Bacteria harboring β-lactamase enzymes [E.C. 3.5.2.6] pose a significant threat to public health. These enzymes prevent β-lactam antibiotics from reaching their intended target, the penicillin binding proteins (PBPs). Sulbactam, tazobactam and clavulanic acid are mechanism-based inactivators as they share similarities with the β-lactam structure, the normal substrate for β-lactamases. Similar to a substrate, these inhibitors can, after acylation at catalytic residue S70, undergo several inhibitory reaction pathways including fragmentation in the active site and covalently cross-linking at S130.

Lastly, we changed the position of the ester bond, shortening the tail, and replaced the terminal carboxylate group with an amine group to result in PSR-3-226. PSR-3-226 was also not able to be trapped in the wt SHV-β-lactamase; we suspect that the tail of PSR-3-226 is not capable of forming a trans-enamine stabilizing U-shaped conformation. This prompted us to use the deacylation-deficient E166A variant of SHV-1 as we had done previously with difficult to capture compounds. Soaking E166A SHV-1 crystals for 30 minutes with PSR-3-226 yielded a 1.22Å resolution acyl-enzyme structure. Fo-Fc and 2Fo-Fc electron maps and subsequent crystallographic refinement indicated the presence of a covalently-bound partial PSR-3-226 fragment (refined at 100% occupancy) and a nearby HEPES buffer molecule fragment (refined at 80% occupancy). The PSR-3-226 inhibitor fragment, which consists of six atoms, was covalently bound to S70 in a trans-enamine conformation (torsion angle of 175°). Since only six atoms of the inhibitor fragment were able to be resolved, there were few hydrogen bonds observed in the active site; the inhibitor carbonyl oxygen occupied the oxyanion hole, as in SA2-13- and PSR-4-157-bound SHV-1, within hydrogen bonding distance of the mainchain nitrogens of residues A237 and S70. The one exception was residue 166, which was substituted to an alanine from glutamate to capture the inhibitor intermediate. This E166A change resulted in a local distortion of the main chain for this residue similar to what we observed previously for deacylation-deficient E166A inhibitor complexes. Interestingly, PSR-3-226 in both SHV-1 and KPC-2 is accompanied by a nearby buffer molecule interacting in the carboxyl binding pocket.

> SPQPLEQIKLSESQLSGRVGMIEMDLASGRTLTAWRADERFPMMSTFKVVLCGAVLARVDAGDEQLERKIHYRQQDLVDYSPVSEKHLADGMTVGELCAAAITMSDNSAANLLLATVGGPAGLTAFLRQIGDNVTRLDRWATELNEALPGDARDTTTPASMAATLRKLLTSQRLSARSQRQLLQWMVDDRVAGPLIRSVLPAGWFIADKTGAGERGARGIVALLGPNNKAERIVVIYLRDTPASMAERNQQIAGIGAALIEHWQR> DLEDL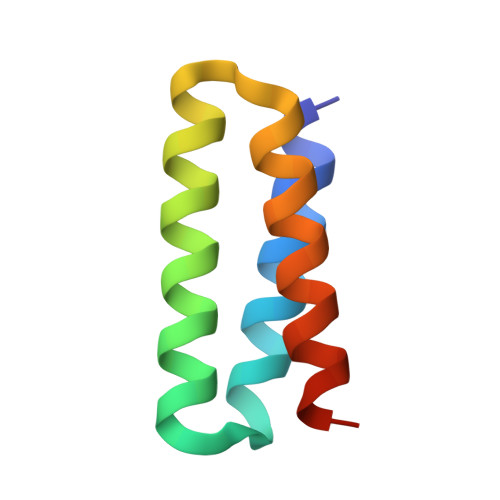LEKIKDIVLKVMDIGDDETIKRAQKLLIKAELAVENKDLKEVEKLLKEAEKVYKEVKEAK> SGDYRVQNTSLEAIVQNASSDNQGIQLSAVQAARKLLSSDRNPPIDDLIKSGILPILVHCLERDDNPSLQFEAAWALTNIASGTSEQTQAVVQSNAVPLFLRLLHSPHQNVCEQAVWALGNIIGDGPQCRDYVISLGVVKPLLSFISPSIPITFLRNVTWVMVNLCRHKDPPPPMETIQEILPALCVLIHHTDVNILVDTVWALSYLTDAGNEQIQMVIDSGIVPHLVPLLSHQEVKVQTAALRAVGNIVTGTDEQTQVVLNCDALSHFPALLTHPKEKINKEAVWFLSNITAGNQQQVQAVIDANLVPMIIHLLDKGDFGTQKEAAWAISNLTISGRKDQVAYLIQQNVIPPFCNLLTVKDAQVVQVVLDGLSNILKMAEDEAETIGNLIEECGGLEKIEQLQNHENEDIYKLAYEIIDQFFSSDDIDEDPSLVPEAIQGGTFGFNSSANVPTEGFQF;> SRNIHLLGRKTCLGRRVVQPGMFEDHPPTKKARVSMRRMSN

Active transport of proteins from the cytoplasm to the nucleus is mediated by a family of nuclear transport receptors known as importins (or karyopherins), together with a number of ancillary proteins including nucleoporins and Ran1–3. Importin α is constructed from an N-terminal importin β-binding (IBB) domain and a C-terminal NLS binding domain featuring ten armadillo (ARM)-repeat motifs. The W proteins of henipaviruses share a common N-terminal domain with P and V proteins, but have a unique NLS bearing C-terminal domain that is recognised preferentially by importins α3 and α4 (KPNA4 and KPNA3), rather than the better characterised importin α1 (KPNA2). In this study, we present high-resolution structures of importin α isoform adaptors bound to the NLS regions of HeV W and NiV W, providing insights into the molecular basis of importin α isoform specificity.

To test whether the same binding patterns were present in the NiV W protein, we examined the binding determinants of importin α:NiV W complexes using the same approach. We observed binding patterns that were very similar to those seen with HeV W for both importin α1 and α3. In comparison, the importin α3:NiV W complex had P1211 symmetry, diffracted to 2.3 Å resolution, and showed more extensive binding, with residues 421–446 bound to importin α3. The importin α3:NiV W interface was mediated through 31 hydrogen bonds, seven salt bridge interactions, and buried 1591.8 Å2 of surface area. However, there were marked differences residing outside this region, with importin α3 ARM repeats 6–9 binding HeV W and NiV W residues 419–444 and 421–446, respectively. Notably, despite binding the same region of HeV W and NiV W, importin α3 exhibited a 2.4-fold more extensive interaction buried surface area than importin α1, with 16 additional hydrogen bonds, and six additional salt bridge interactions, consistent with its > 50-fold higher affinity. We found that mutations within the viral W proteins predicted to disrupt interactions at the minor site of importin α3 (specifically, R422A/R423A and R422D/R423D in the HeV W C-terminal domain and R424A/R425A and R424D/R425D in NiV W C-terminal domain) were no longer pulled down with importin α3 in our co-immunoprecipitation assay. Similarly, mutations predicted to disrupt interaction at the importin α3 major site, K437A/K438A and K437D/K438D in HeV W C-terminal domain, and K439A/K440A and K439D/K440D in the NiV W C-terminal domain, also failed to interact with importin α3. To further test the involvement of ARMs 7 and 8 in mediating specificity, we designed an importin α3 mutant based on the structural data to disrupt interactions in ARMs 7/8 (N348 A/N352A/E387A/N394A), and found a marked reduction in binding to both HeV and NiV W proteins. We found that the isoform specificity was localised to the C-terminal ARM repeats 7 and 8, and that the positioning of these domains was an important determinant for mediating specificity.> MATKGTKRSYEQMETDGERQNATEIRASVGKMIDGIGRFYIQMCTELKLSDYEGRLIQNSLTIERMVLSAFDERRNKYLEEHPSAGKDPKKTGGPIYRRVDGKWRRELILYDKEEIR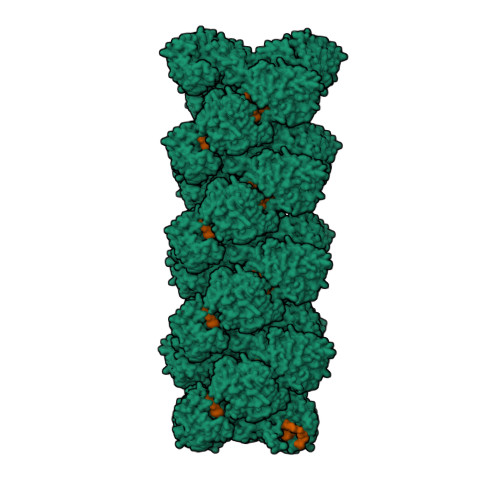RIWRQANNGDDATAGLTHMMIWHSNLNDATYQRTRALVRTGMDPRMCSLMQGSTLPRRSGAAGAAVKGVGTMVMELIRMIKRGINDRNFWRGENGRRTRIAYERMCNILKGKFQTAAQRTMVDQVRESRNPGNAEFEDLIFLARSALILRGSVAHKSCLPACVYGSAVASGYDFEREGYSLVGIDPFRLLQNSQVYSLIRPNENPAHKSQLVWMACHSAAFEDLRVSSFIRGTKVVPRGKLSTRGVQIASNENMETMESSTLELRSRYWAIRTRSGGNTNQQRASSGQISIQPTFSVQRNLPFDRPTIMAAFTGNTEGRTSDMRTEIIRLMESARPEDVSFQGRGVFELSDEKATSPIVPSFDMSNEGSYFFGDNAEEYDNLEHHHHHH> GSMGDTKEQRILRYVQQNAKPGDPQSVLEAIDTYCTQKEWAMNVGDAKGQIMDAVIREYSPSLVLELGAYCGYSAVRMARLLQPGARLLTMEMNPDYAAITQQMLNFAGLQDKVTILNGASQDLIPQLKKKYDVDTLDMVFLDHWKDRYLPDTLLLEKCGLLRKGTVLLADNVIVPGTPDFLAYVRGSS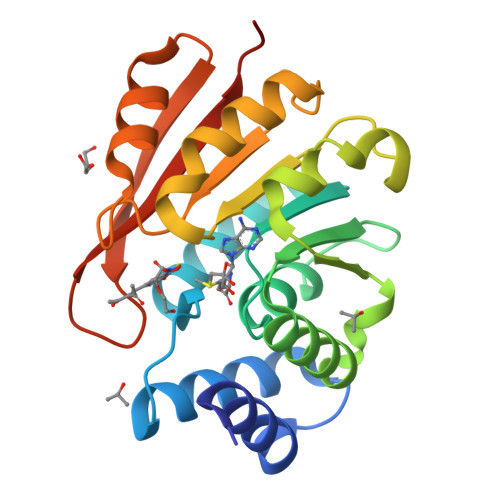SFECTHYSSYLEYMKVVDGLEKAIYQGPSSPDKS>[2x]GSMYQLQFINLVYDTTKLTHLEQTNINLFIGNWSNHQLQKSICIRHGDDT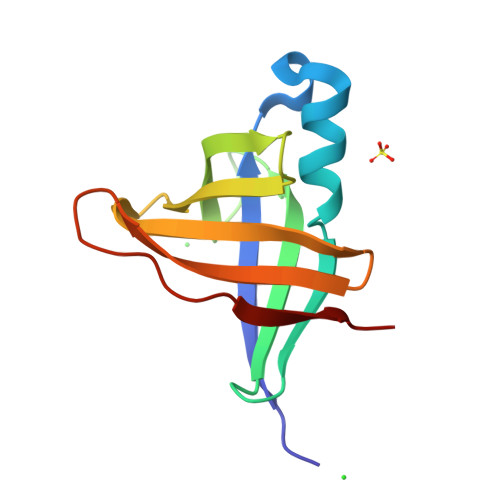SHNQYHILFIDTAHQRIKFSSFDNEEIIYILDYDDTQHILMQTSSKQGIGTSRPIVYERLV> MPDTSFSNPGLFTPLQLGSLSLPNRVIMAPLTRSRTPDSVPGRLQQIYYGQRAS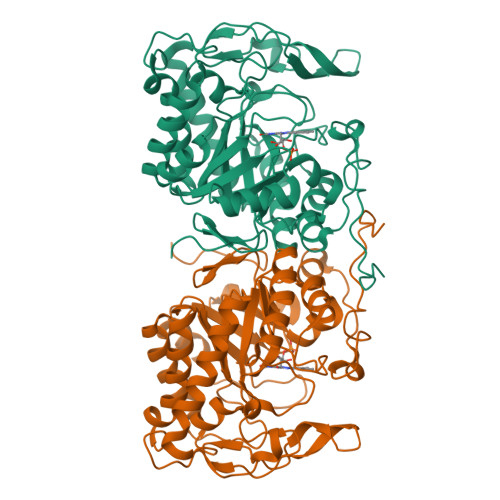AGLIISEATNISPTARGYVYTPGIWTDAQEAGWKGVVEAVHAKGGRIALQLWHVGRVSHELVQPDGQQPVAPSALKAEGAECFVEFEDGTAGLHPTSTPRALETDGIPGIVEDYRQAAQRAKRAGFDMVEVHAANACLPNQFLATGTNRRTDQYGGSIENRARFPLEVVDAVAEVFGPERVGIRLTPFLELFGLTDDEPEAMAFYLAGELDRRGLAYLHFNEPDWIGGDITYPEGFREQMRQRFKGGLIYCGNYDAGRAQARLDDNTADAVAFGRPFIANPDLPERFRLGAALNEPDPSTFYGGAEVGYTDYPFLDNGHDRLG>MLNRVVLVGRLTKDPEYRTTPSGVSVATFTLAVNRTFTNAQGEREADFINCVVFRRQADNVNNYLSKGSLAGVDGRLQSRNYENQEGRRVFVTEVVCDSVQFLEPKHHHHHH[2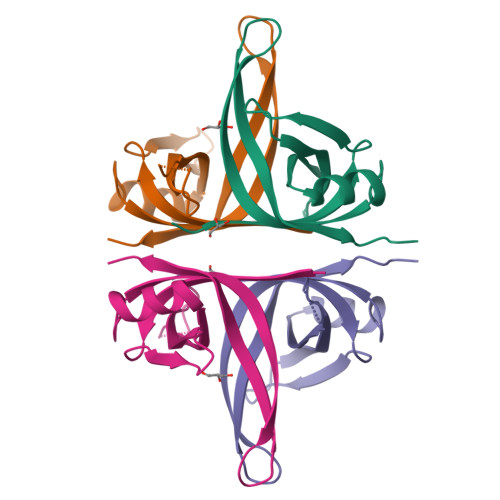x]> KKIFKPEELRQALMPTLEALYRQDPESLPFRQPVDPQLLGIPDYFDIVKSPMDLSTIKRKLDTGQYQEPWQYVDDIWLMFNNAWLYNRKTSRVYKYCSKLSEVFEQEIDPVMQSLGYCCGRKLEFSPQTLCCYGKQLCTIPRDATYYSYQNRYHFCEKCFNEIQGESVSLGDDPSQPQTTINKEQFSKRKNDTLDPELFVECTECGRKMHQICVLHHEIIWPAGFVCDGCLKKSARTRKENKFSAKRLPSTRLGTFLENRVNDFLRRQNHPESGEVTVRVVHASDKTVEVKPGMK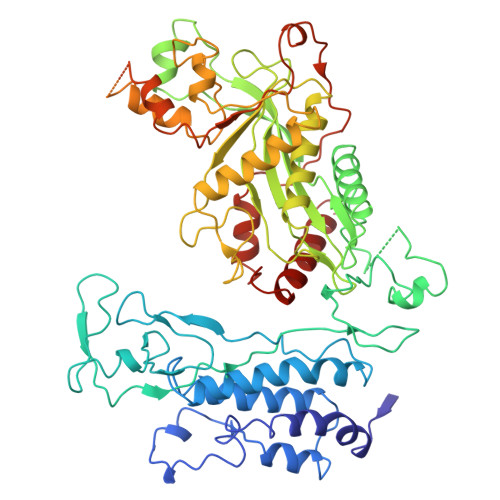ARFVDSGEMAESFPYRTKALFAFEEIDGVDLCFFGMHVQEYGSDCPPPNQRRVYISYLDSVHFFRPKCLRTAVYHEILIGYLEYVKKLGYTTGHIWACPPSEGDDYIFHCHPPDQKIPKPKRLQEWYKKMLDKAVSERIVHDYKDIFKQATEDRLTSAKELPYFEGDFWPNVLEESIKELEQEEEERKREENTSNESTDVTKGDSKNAKKKNNKKTSKNKSSLSRGNKKKPGMPNVSNDLSQKLYATMEKHKEVFFVIRLIAGPAANSLPPIVDPDPLIPCDLMDGRDAFLTLARDKHLEFSSLRRAQWSTMCMLVELHTQSQD>MGHHHHHHVIQWYPGHMAKAKREVSEQLKKVDVVFELVDARIPYSSRNPMIDEVINQKPRVVILNKKDMSNLNEMSKWEQFFIDKGYYPVSVDAKHGKNLKKVEAAAIKATAEKFEREKAKGLKPRAIRAMIVGIPNVGKSTLINKLAKRSIAQTGNKPGVTKQ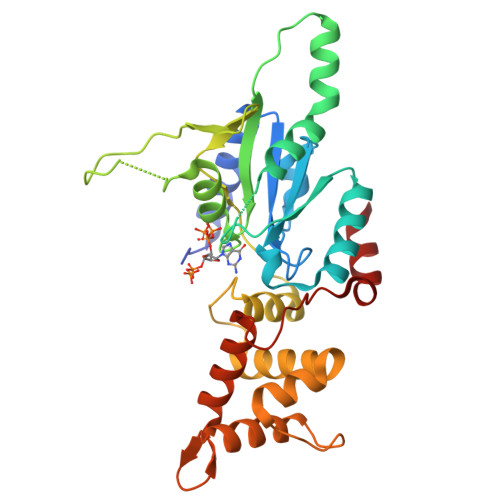QQWIKVGNALQLLDTPGILWPKFEDEEVGKKLSLTGAIKDSIVHLDEVAIYGLNFLIQNDLARLKSHYNIEVPEDAEIIAWFDAIGKKRGLIRRGNEIDYEAVIELIIYDIRNAKIGNYCFDIFKDMTEELANDANN[2x]(3~{a}~{R},4~{R},5~{S},6~{R},7~{R},7~{a}~{S})-7-(hydroxymethyl)-2,2-bis(oxidanylidene)-3~{a},4,5,6,7,7~{a}-hexahydrobenzo[d][1,3,2]dioxathiole-4,5,6-triol | C7 H12 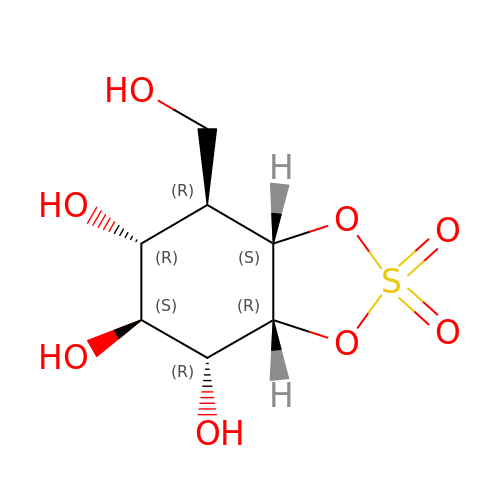O8 S | ZCXRKCCKXOHKLN-XQCVOTFFSA-N> TKRFYVKDHRNKAMINLHIQKDNPKIVHAFDMEDLGDKAVYCRCWRSKKFPFCDGAHTKHNEETGDNVGPLIIKKKET

MitoNEET (gene cisd1) was identified in 2004 as the first example of a mitochondrial outer-membrane iron–sulfur protein, with the cluster binding domain facing the cytosolic side1. This protein was initially discovered as the unintended target for the anti-diabetic peroxisome proliferator-activated receptor gamma (PPAR-γ) agonist pioglitazone, as many of the beneficial effects of pioglitazone, a thiazolidinedione (TZD), could not be explained by PPAR-γ activity alone. MitoNEET assembles as a homodimer, with each subunit containing a rather unusual [2Fe–2S]-type iron–sulfur cluster coordinated by His87 and three cysteine residues2. The amino acids coordinating the [2Fe–2S] cluster form a signature CDGSH domain common to all members of the CISD-gene family.

Here, we present the first crystal structure at 1.95 Å resolution of human mitoNEET with a bound benzoic-sulfonamide-furan ligand, furosemide. We focused on furosemide in this study due to its appropriateness for the X-ray diffraction studies, due to its favorable solubility profile, as opposed to the glitazones where solubility in the crystallization mother liquor is limiting. In the refined structure, furosemide is bound on the face close to the [2Fe–2S] cluster in each monomer, which are critical for the biological function of mitoNEET. The bound ligand was supported by strong density after MR-SAD phasing and refinement, and was further confirmed by simulated annealing OMIT map analysis. The furosemide carboxylic groups are in reach of the [2Fe–2S] coordinating His87 side chain for possible hydrogen bonding with His87Nε. In addition, the furan ring of furosemide can be modeled such that the oxygen is pointed toward Sγ of the Cys83 ligand, although the limited resolution of the refined electron density map cannot discriminate the precise orientation of the furosemide furan ring in the present study. The furosemide-binding site observed in the crystal structure corresponds to previously hypothesized binding pocket, from molecular docking studies performed with the anticancer drug MAD-28 corroborating our finding. In accordance, the Phe82 side chain is within a 5 Å distance from the furosemide furan ring in the refined structure, which could suggest that this is the same binding site that pioglitazone occupies. Considering also the previous report that pioglitazone inhibits cluster release from mitoNEET under oxidative stress, it seems likely that the compounds binding in the furosemide pocket would stabilize the ligation environment of the [2Fe–2S] cluster. The primary binding site identified correlates with the redox-active [2Fe–2S] cluster ligation site, and binding to the HIS87 and LYS55 may inhibit its redox function and/or possible cluster release/breakdown at the cytoplasmic side.>MKSLGRHLVAEFYECDREVLDNVQLIEQEMKQAAYESGATIVTSTFHRFLPYGVSGVVVISESHLTIHTWPEYGYAAIDLFTCGEDVDPWKAFEHLKKALKAKRVHVVEHERGRYDEIGIPEDSPHK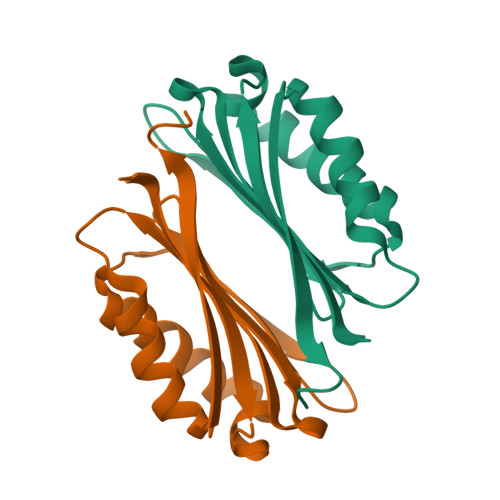AAV[2x]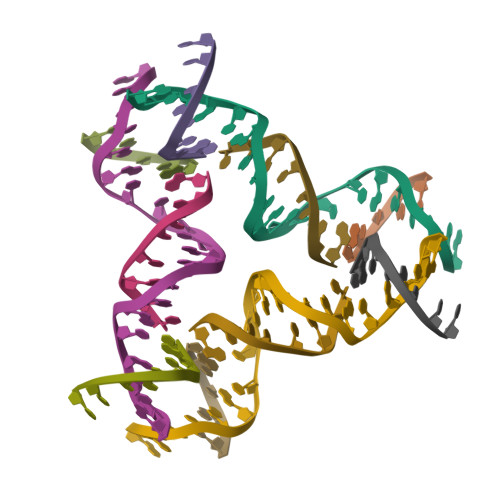> GAGCAGCTGTGACGGACATCA;> CCGTCACA;> GCTGC;> TCTGATGT>RFLKVKNWETDVVLTDTLHLKSTLETGCTEHICMGSIMLPSQHTRKPEDVRTKDQLFPLAKEFLDQYYSSIKRFGSKAHMDRLEEVNKEIESTSTYQLKDTELIYGAKHAWRNASRCVGRIQWSKLQVFDARDCTTAHGMFNYICNHVKYATNKGNLRSAITIFPQRTDGKHDFRVWNSQLIRYAGYKQPDGSTLGDPANVQFTEICIQQGWKAPRGRFDVLPLLLQANGNDPELFQIPPELVLEVPIRHPKFDWFKDLGLKWYGLPAVSNMLLEIGGLEFSACPFSGWYMGTEIGVRDYCDN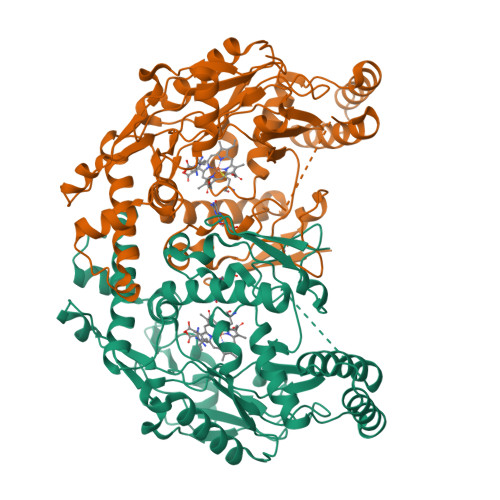SRYNILEEVAKKMDLDMRKTSSLWKDQALVEINIAVLYSFQSDKVTIVDHHSATESFIKHMENEYRCRGGCPADWVWIVPPMSGSITPVFHQEMLNYRLTPSFEYQPDPWNTHVWKG[2x]> HHHHHHSGNTLKIEAESYLYSNDVQKEPCSEGGENVGYINNGSWMSYPGINFPSSGNYLIEYRVASAVDGGRFSSDLEAGETVLGELSVPNTGGWQNWTTVSQTVNV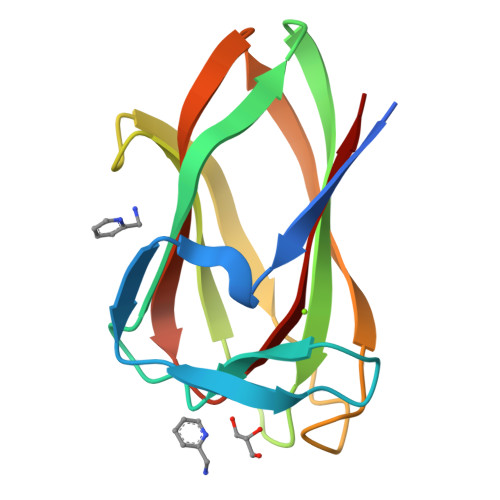SAGTYQFGLYSISGGWNINWIRITK> QDNSRYTHFLTQHYDAKPQGRDDRYCESIMRRRGLTSPCKDINTFIHGNKRSIKAICENKNGNPHRENLRISKSSFQVTACKLHGGSPWPPCQYRATAGFRNVVVACENGLPVHLD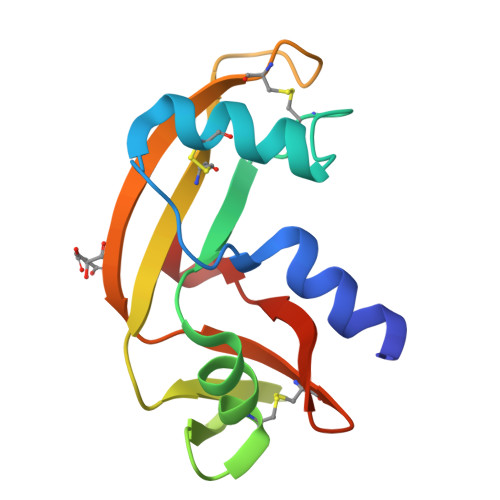QSIFRRP> GPHMSLTVKAYLLGKEDAAREIRRFSFCCSPEPEAEAEAAAGPGPCERLLSRVAALFPALRPGGFQAHYRAERGDLVAFSSD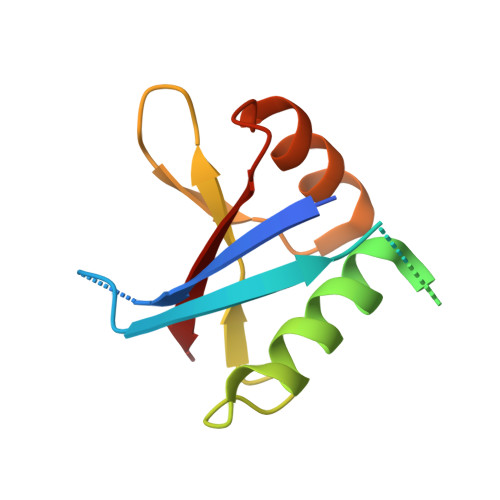EELTMAMSYVKDDIFRIYIKEK> QLSGSVGPLTSASTKGATKTCNILSYGAVADNSTDVGPAITSAWAACKSGGLVYIPSGNYALNTWVTLTGGSATAIQLDGIIYRTGTASGNMIAVTDTTDFELFSSTSKGAVQGFGYVYHAEGTYGARILRLTDVTHFSVHDIILVDAPAFHFTMDTCSDGEVYNMAIRGGNEGGLDGIDVWGSNIWVHDVEVTNKDECVTVKSPANNILVESIYCNWSGGCAMGSLGADTDVTDIVYRNVYTWSSNQMYMIKSNGGSGTVSNVLLENF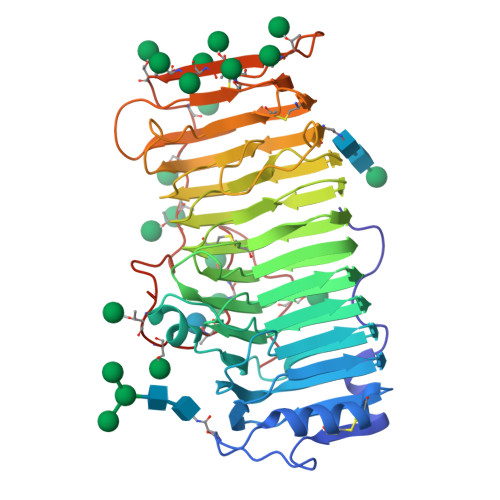IGHGNAYSLDIDGYWSSMTAVAGDGVQLNNITVKNWKGTEANGATRPPIRVVCSDTAPCTDLTLEDIAIWTESGSSELYLCRSAYGSGYCLKDSSSHTSYTTTSTVTAAPSGYSATTMAADLATAFGLTASIPIPTIPTSFYPGLTPYSALAG>MAGWQSYVDNLMCDGCCQEAAIVGYCDAKYVWAATAGGVFQSITPVEIDMIVGKDREGFFTNGLTLGAKKCSVIRDSLYVDGDCTMDIRTKSQGGEPTYNVAVGRAGRVLVFVM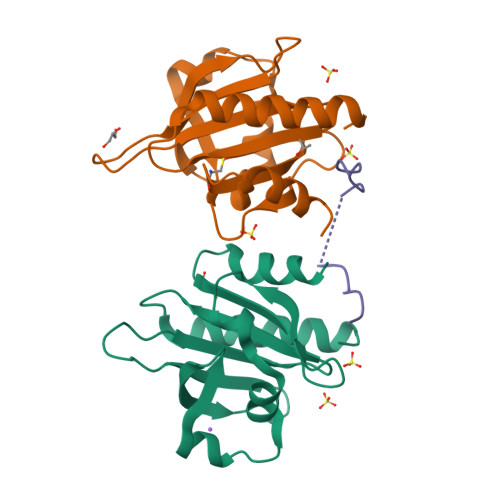GKEGVHGGGLNKKAYSMAKYLRDSGF[2x];> IPPPPPLPGVASIPPPPPLPG> MASMTGGQQMGRDEAGITGTWYNQLGSTFIVTAGADGALTGTYESAVGNAESRYVLTGRYDSAPATDGSGTALGWTVAWKNNYRNAHSATTWSGQYVGGAEARINTQWLLTMGTTEANAWASTLVGHDTFTKVKPSAASIDAAKKAGVNNGNP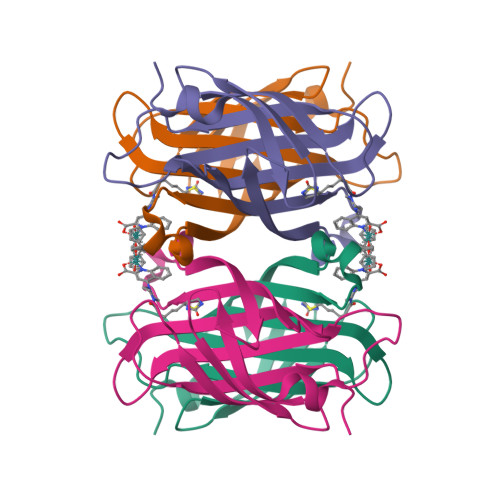LDAVQQ HISTIDINE-METHYL-ESTER | C7 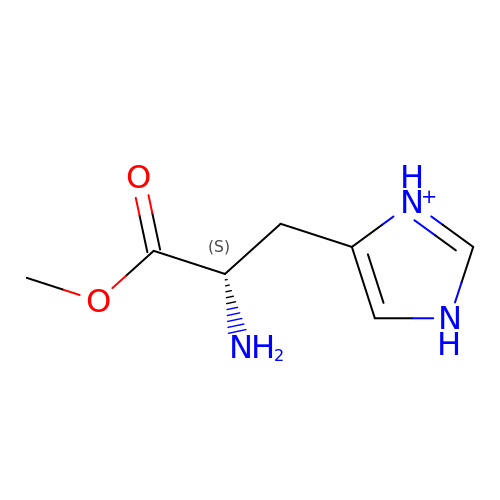H12 N3 O2 | BXRMEWOQUXOLDH-LURJTMIESA-O>MGSSHHHHHHSSGLVPRGSMESGFTSKDTYLSHFNPRDYLEKYYKFGSRHSAESQILKHLLKNLFKIFCLDGVKGDLLIDIGSGPTIYQLLSACESFKEIVVTDYSDQNLQELEKWLKAAPAAFDWSPVVTYVCDLEGNRVKGPEKEEKLRQAVKQVLKCDVTQSQPLGAVPLPPADCVLSTLCLDAACPDLPTYCRALRNLGSLLKPGGFLVIMDALKSSYYMIGEQKFSSLPLGREAVEAAVKEAGYT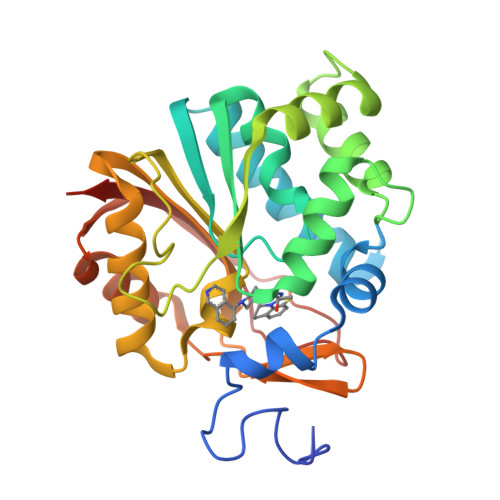IEWFEVISQSYSSTMANNEGLFSLVARKLSRPL[4x]> MEKYNPHAIEAKWQRFWEEKGFMKAKDLPGGRGKQYVLVMFPYPSGDLHMGHLKNYTMGDVLARFRRMQGYEVLHPMGWDAFGLPAENAALKFGVHPKDWTYANIRQAKESLRLMGILYDWDREVTTCEPEYYRWNQWIFLKMWEKGLAYRAKGLVNWCPKCQTVLANEQVVEGRCWRHEDTPVEKRELEQWYLRITAYAERLLKDLEGLNWPEKVKAMQRAWIGRSEGAEILFPVEGKEVRIPVFTTRPDTLFGATFLVLAPEHPLTLELAAPEKREEVLAYVEAAKRKTEIERQAEGREKTGVFLGAYALNPATGERIPIWTADYVLFGYGTGAIMAVPAHDQRDYEFARKFGLPIKKVIERPGEPLPEPLERAYEEPGIMVNSGPFDGTESEEGKRKVIAWLEEKGLGKGRVTYRLRDWLISRQRYWGTPIPMVHCEACGVVPVPEEELPVLLPDLKDVEDIRPKGKSPLEAHPEFYETTCPKCGGPAKRDTDTMDTFFDSSWYYLRYTDPHNDRLPFDPEKANAWMPVDQYIGGVEHAVLHLLYSRFFTKFLHDLGMVKVEEPFQGLFTQGMVLAWTDFGPVEVEGSVVRLPEPTRIRLEIPESALSLEDVRKMGAELRPHEDGTLHLWKPAVMSKSKGNGVMVGPFVKEQ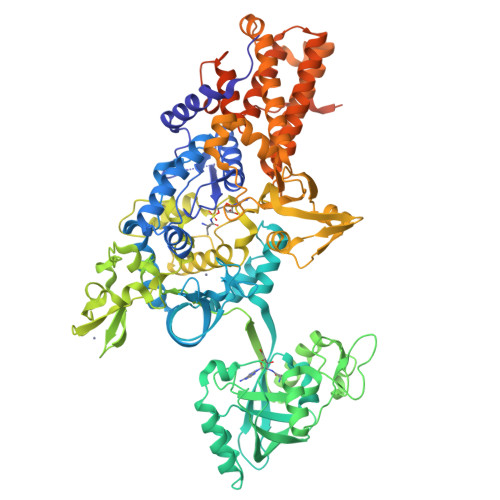GADIARITILFAAPPENEMVWTEEGVQGAWRFLNRIYRRVAEDREALLETSGVFQAEALEGKDRELYGKLHETLKKVTEDLEALRFNTAIAALMEFLNALYEYRKDRPVTPVYRTAIRYYLQMLFPFAPHLAEELWHWFWPDSLFEAGWPELDEKALEKDVVEVAVQVNGRVRGTIHIPKDAPLEVARAEALKVRNVRAHLEGKEVVKEIYVPGKILNLVVRG> MQRLFLLVAVMLLSGCLTAPPKEAARPTLMPRAQSYKDLTHLPAPTGKIFVSVYNIQDETGQFKPYPASNFSTAVPQSATA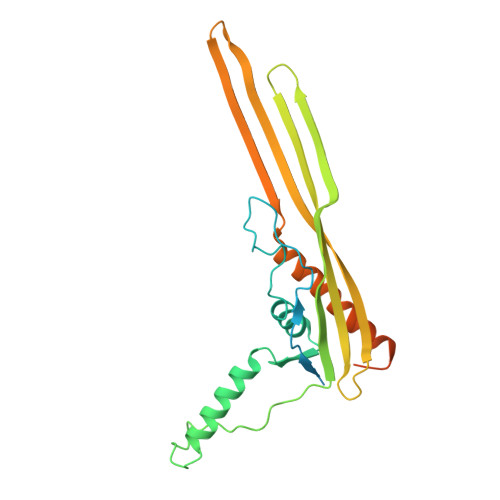MLVTALKDSRWFIPLERQGLQNLLNERKIIRAAQENGTVAINNRIPLQSLTAANIMVEGSIIGYESNVKSGGVGARYFGIGADTQYQLDQIAVNLRVVNVSTGEILSSVNTSKTILSYEVQAGVFRFIDYQRLLEGEVGYTSNEPVMLCLMSAIETGVIFLINDGIDRGLWDLQNKAERQNDILVKYRHMSVPPESWSHPQFEK>MRITFNDVKTSLGITESYDIVNAIRNSQGDNFKSYVPLATANNVAEVGAGILINQTVQNDFITSLVDRIGLVVIRQVSLNNPLKKFKKGQIPLGRTIEEIYTDITKEKQYDAEEAEQKVFEREMPNVKTLFHERNRQGFYHQTIQDDSLKTAFVSWGNFESFVSSIINAIYNSAEVDEYEYMKLLVDNYYSKGLFTTVKIDEPTSSTGALTEFVKKMRATARKLTLPQGSRDWNSMAVRTRSYMEDLHLIIDADLEAELDVDVLAKAFNMNRTDFLGN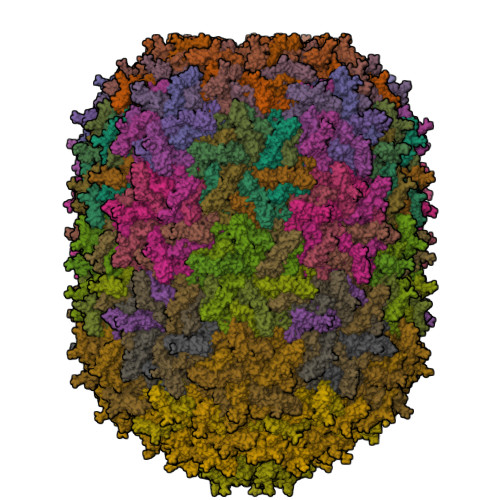VTVIDGFASTGLEAVLVDKDWFMVYDNLHKMETVRNPRGLYWNYYYHVWQTLSVSRFANAVAFVSGDVPAVTQVIVSPNIAAVKQGGQQQFTAYVRATNAKDHKVVWSVEGGSTGTAITGDGLLSVSGNEDNQLTVKATVDIGTEDKPKLVVGEAVVSIRPNNASGGAQA[47x]>[2x]GHMVTRIENLENAKKLWDNANSMLEKGNISGYLKAANELHKFMKEKNLKEDDLRPELSDKTISPKGYAILQSLWGAASDYSRAAATLTESTVEPG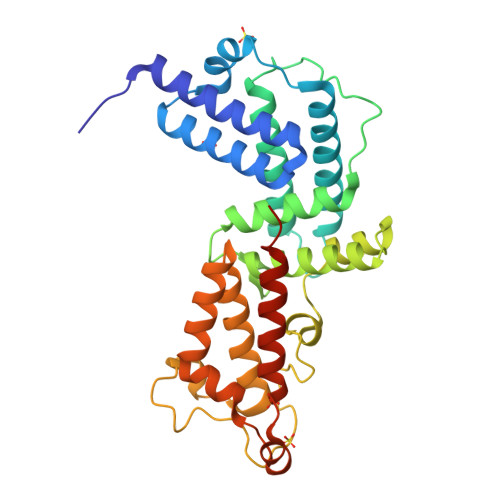LVSAVNKMSAFFMDCKLSPNERATPDPDFKVGKSKILVGIMQFIKDVADPTSKIWMHNTKALMNHKIAAIQKLERSNNVNDETLESVLSSKGENLSEYLSYKYATKDEGREHRYTASTENFKNVKEKYQQMRGDALKTEILADFKDKLAEATDEQSLKQIVAELKSKDEYRILAKGQGLTTQLLGLKTSSVSSFEKMVEETRESIKSQERQTIKIK> MSTQTEVPAPQPKKTRRRTLYRGDPGMWSWVLHRITGATIFFFLFVHVLDTALVRVSPQAYNEVIETYKTPIVGLMEIGLVAAVLFHALNGIRVILIDF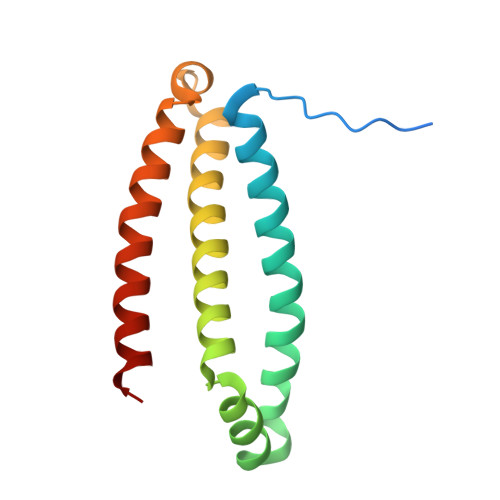WAKGPRYQRQMLAVIAGLFLVIFIAAVGVIGMHMVERFL>[9x]FAQLDNSKPFKIKDITRNIRKAVVATTISEIRTKVSLKFERAQRRIHLDC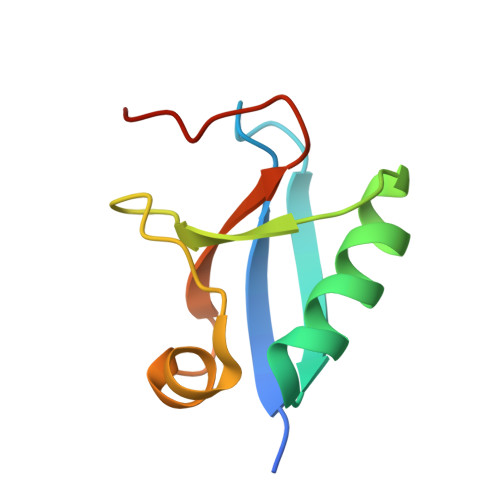DGTEVDDEEYFSTLEPNAELIAVFPGEQWRDPSD> MMPQWAYMHIAGQDASEYLSPGLVQFARATDTYFSLGNKFRNPTVAPTHDVTTDRSQRLTLRFVPVDREDTTYSYKARFTLAVGDNRVLDMASTYFDIRGVLDRGPSFKPYSGTAYNSLAPKSAPNPSQWTANEKQTGGQPKSVTQTFGSAPMGGSN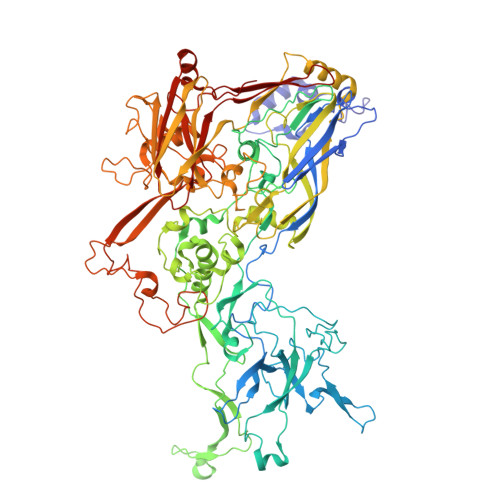ITIEGLVIGTKEEEGNATEEIFADKTFQPEPQVGEENWQETEAFYGGRALKKDTKMKPCYGSFARPTNEKGGQAKLKLNDQGQPTKDYDIDLAFFDTPGGTPPTGSGQQEEYKADIVMYTENVNLETPDTHVVYKPGKEDESSETNLTQQSMPNRPNYIGFRDNFVGLMYYNSTGNMGVLAGQASQLNAVVDLQDRNTELSYQLLLDSLGDRTRYFSMWNSAVDSYDPDVRIIENHGVEDELPNYCFPLNGTGTNSTYQGVKVKTGQDGAEETEWDKDETVARQNQIAKGNVYAMEINLQANLWKSFLYSNVALYLPDSYKYTPANVTLPANTNTYEYMNGRVVAPSLVDAYINIGARWSLDPMDNVNPFNHHRNAGLRYRSMLLGNGRYVPFHIQVPQKFFAIKNLLLLPGSYTYEWNFRKDVNMILQSSLGNDLRVDGASVRFDSVNLYATFFPMAHNTASTLEAMLRNDTNDQSFNDYLSAANMLYPIPAKATNVPISIPSRNWAAFRGWSFTRLKTKETPSLGSGFDPYFVYSGSIPYLDGTFYLNHTFKKVSIMFDSSVSWPGNDRLLTPNEFEIKRSVDGEGYNVAQCNMTKDWFLVQMLSHYNIGYQGFHVPEGYKDRMYSFFRNFQPMSRQVVDEINYKDYKAVTLPFQHNNSGFTGYLAPTMRQGQPYPANFPYPLIGQTAVPSVTQKKFLCDRVMWRIPFSSNFMSMGALTDLGQNMLYANSAHALDMTFEVDPMDEPTLLYLLFEVFDVVRVHQPHRGVIEAVYLRTPFSAGN> GHMMVKIMPNLPGLYFLQAYPSEEIWRLFVDGRFWSKENGWRGYESREPGSLNAALESLCSIALQVEKSGEEFELSVDLIKRIHKKSGKKVEELQEKNPGELRTDEPVSFCIPAGRASIKGIEEFLSLVFLTEGGAEFGPGKAGPFGPRFDKNYFKNLNPEQIPDLAKQIYFDMSKYGHSNTNHFYLAVMKNVDVYLEKITQSYNKEIKTAETLDEKLKIIVKHIRMYEVLHPFRDANGRTFVNNLLNILLMQQGLPPATFYEPNVFDLYSAEELVVVVKEAIFNTVEIIEQSKRKTPITLYGYHSSLEEQTKFRDMLDSPSYEKIKHMDFSDLNPEKLHLKTQKCLSSLNEQYPLHRGAIYLSDPGEIKLLLSNRNESQINQQIEQGAPPIYVGKTPAHLAVISGNMAMLDELIAKKADLSLQDYDGKTALHYAAECGNMQIMGKILKVVLSQEDAIKVLNIKDNHGKTAFHYAAEFGTPELISALTTTEVIQINEPDNSGSSAITLAYKNHKLKIFDELLNSGADISDELLDAIWARKDKETLGKIIAKNEKILLNKEAFRIAISLGSVSLVKKFLRAGVDIDIPLTKDKATPLMLSINSGNPKLVSYLLKKGANTRLTDTSGNSVLHYVFYSKAENREALANIITEKDKKLINQPNANGNPPLYNAVVVNDLKMATILLEMGARVDFEDRLGNNILHSAMRRCDLPIILDIVKKDSTLLHKRNSERRNPFHQALHEMHTFPSSKETEEIHFMNLSDLLLKEGVDLNKKDIKGKTILDIALSKQYFHLCVKLMKAGAHTNI;> GPMPEYDYLFKLLLIGDSGVGKSCLLLRFADDTYTESYISTIGVDFKIRTIELDGKTIKLQIWDTAGQERFRTITSSYYRGAHGIIVVYDVTDQESYANVKQWLQEIDRYASENVNKLLVGNKSDLTTKKVVDNTTAKEFADSLGIPFLETSAKNATNVEQAFMTMAAEIKKRMG

The causative agent of Legionnaires disease, Legionella pneumophila, translocates the phosphocholine transferase AnkX during infection and thereby posttranslationally modifies the small guanosine triphosphatase (GTPase) Rab1 with a phosphocholine moiety at S76 using cytidine diphosphate (CDP)–choline as a cosubstrate. AnkX contains 949 amino acids and two individual structural units: The N terminus (amino acids 1 to 350) is constituted by a FIC [filamentation induced by cyclic adenosine monophosphate (AMP)] domain that contains the CDP-choline binding pocket. In addition, the amino acid region 351 to 800 forms an ankyrin repeat (AR) domain with currently unknown function. Rab proteins function as molecular switches in cellular signaling and alternate between inactive guanosine diphosphate (GDP)–bound and active guanosine trisphosphate (GTP)–bound states.

We therefore developed a strategy to covalently capture Rab1b with AnkX via its nucleotide cosubstrate, thus allowing us to characterize the AnkX:Rab1b:PC complex by x-ray crystallography. AnkX1–800 reveals a scoop-like structure that consists of the globular FIC domain (amino acids 1 to 350) and 13 curved ARs (amino acids 351 to 800). Thus, AnkX is forming a cavity in whose center Rab1b is embraced. Whereas ARs 1 to 4 are serving as structural support for the FIC domain ARs 5 to 13 are forming multiple interactions to Rab1b. In Rab1b, no electron density is observed for the amino acids 68 to 74 of the switch II region (amino acids 64 to 83). Although the modified S76Rab1b is ordered in the complex structure, no electron density is observed for PC and the linker between PC and G108CAnkX. However, the switch II loop of Rab1b including S76Rab1b is not reaching into the catalytic pocket of AnkX, indicating that the structure may represent a postcatalytic complex. The crystal structure of AnkXG108C:PC:Rab1b:GDP revealed three interfaces for AnkX binding. F143AnkX is located at the tip of the thorn and binds into a hydrophobic pocket of Rab1b between switch II and α3. AnkX locally unfolds the GTPase switch II by F143AnkX-mediated displacement of Y78Rab1b.>[2x]MAMANNSSVANKVCLIVIDGWGVSEDPYGNAILNAQTPVMDKLCSGNWAQIEAHGLHVGLPEGLMGNSEVGHLNIGAGRVIYQDIVRINLAVKNNKFVTNESLVDACDRAKNGNGRLHLAGLVSDGGVHSHIDHMFALVKAIKELGVPELYLHFYGDGRDTSPNSGVGFLEQTLEFLEKTTGYGKLATVVGRYYAMDRDNRWERINVAYEAMIGGVGETSDEAGVVEVVRKRYAADETDEFLKPIILQGEKGRVQNDDTIIFFDYRADRMREISAAMGMDRYKDCNSKLAHPSNLQVYGMTQYKAEFPFKSLFPPASNKNVLAEWLAEQKVSQFHCAETEKYAHVTFFFNGGLEKQFEGEERCLVPSPKVATYDLQPEMSAAGVADKMIEQLEAGTHPFIMCNFAPPDMVGHTGVYEAAVKACEATDIAIGRIYEATQKHGYSLMVTADHGNAEKMKAPDGGKHTAHTCYRVPLTLSHPGFKFVDPADRHPALCDVAPTVLAI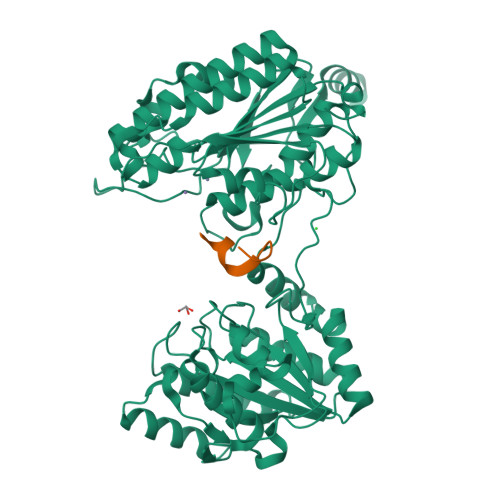MGLPQPAEMTGVSIVQKIKLAAALEHHHHHH;>[2x]XYDYPGDYCYLYX> SHMDYLFKLLLIGDSG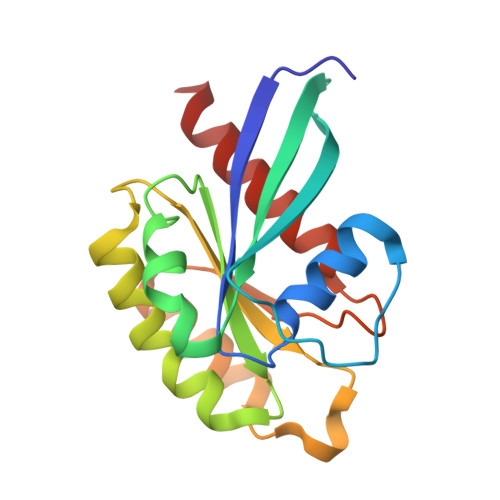VGKTCVLFRFSEDAFNSTFISTIGIDFKIRTIELDGKRIKLQIWDTAGQERFRTITTAYYRGAMGIMLVYDITNEKSFDNIRNWIRNIEEHASADVEKMILGNKCDVNDKRQVSKERGEKLALDYGIKFMETSAKANINVENAFFTLARDIKAKMDKK> GAMDPEFSSDTSHTSKYFGSIDSSENNHKAKMNTGMEESEHFIKCVLQDPIWLLMADADSSVMMTYQLPSRNLEAVLKEDREKLKLLQKLQPRFTESQKQELREVHQWMQTGGLPAAIDVAEC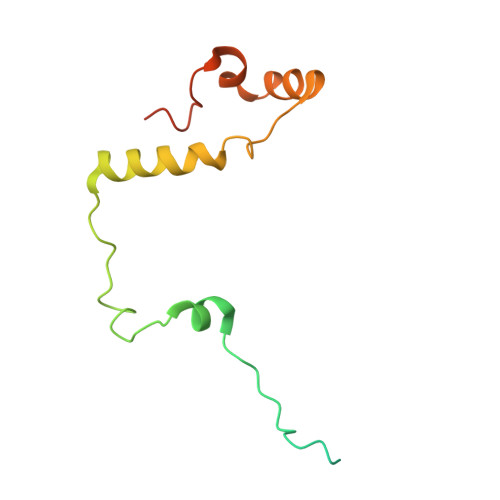VYCES> GELMPPQLQNGLNLSAKVVQGSLDSLPQAVREFLENNAELCQPDHIHICDGSEEENGRLLGQMEEEGILRRLKKYDNCWLALTDPRDVARIESKTVIVTQEQRDTVPIPKTGLSQLGRWMSEEDFEKAFNARFPGCMKGRTMYVIPFSMGPLGSPLSKIGIELTDSPYVVASMRIMTRMGTPVLEALGDGEFVKCLHSVGCPLPLQKPLVNNWPCNPELTLIAHLPDRREIISFGSGYGGNSLLGKKCFALRMASRLAKEEGWLAEHMLVLGITNPEGEKKYLAAAFPSACGKTNLAMMNPSLPGWKVECVGDDIAWMKFDAQGHLRAINPENGFFGVAPGTSVKTNPNAIKTIQKNTIFTNVAETSDGGVYWEGIDEPLASGVTITSWKNKEWSSEDGEPCAHPNSRFCTPASQCPIIDAAWESPEGVPIEGIIFGGRRPAGVPLVYEALSWQHGVFVGAAMRSEATAAAEHKGKIIMHDPFAMRPFFGYNFGKYLAHWLSMAQHPAAKLPKIFHVNWFRKDKEGKFLWPGFGENSRVLEWMFNRIDGKASTKLTPIGYIPKEDALNLKGLGHINMMELFSISKEFWDKEVEDIEKYLVDQVNADLPC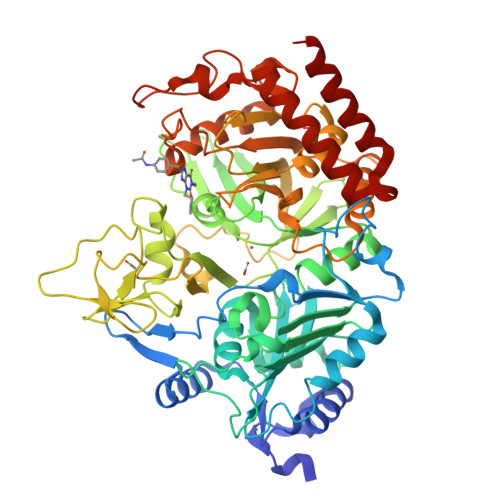EIEREILALKQRISQM> MATLAFILYKYFPFGGLQRDFMRIALECQR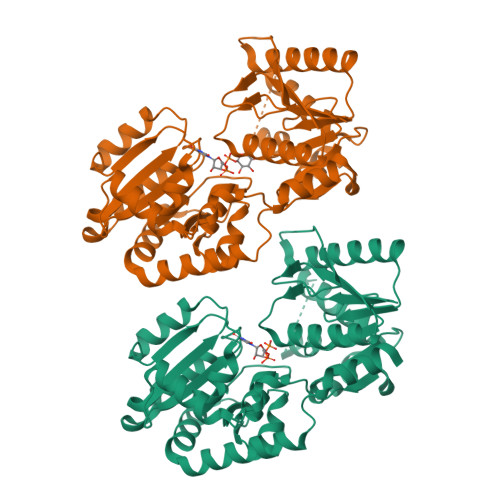RGHDIRVYTLIWEGDVPDGFEVLVAPVRSIFNHRRNEKFTAWVRADLDRRPVQRVIGFNKMPGLDVYYAADACFEEKAQTLRNPLYRQWGRYRHFAGYERAVFDPASKTEILMISEVQQPLFVKHYGTQAERFHLLPPGISQDRRAPANAADVRAEFRREFGLEEDDLLLVQIGSGFKTKGLDRSLKALSALPKALRRRTRLIAIGQDDPKPFLLQIAALGLNDQVQILKGRSDIPRFLLGADLLIHPAYNENTGTVLLEALVSGLPVLVTDVCGYAHYIAEADAGRVLPSPFEQDSLNRLLAEMLEDAPARAAWSRNGLAYADHADLYSMPQRAADLILGEAS;> ATLAFILYKYFPFGGLQRDFMRIALECQRRGHDIRVYTLIWEGDVPDGFEVLVAPVRSIFNHRRNEKFTAWVRADLDRRPVQRVIGFNKMPGLDVYYAADACFEEKAQTLRNPLYRQWGRYRHFAGYERAVFDPASKTEILMISEVQQPLFVKHYGTQAERFHLLPPGISQDRRAPANAADVRAEFRREFGLEEDDLLLVQIGSGFKTKGLDRSLKALSALPKALRRRTRLIAIGQDDPKPFLLQIAALGLNDQVQILKGRSDIPRFLLGADLLIHPAYNENTGTVLLEALVSGLPVLVTDVCGYAHYIAEADAGRVLPSPFEQDSLNRLLAEMLEDAPARAAWSRNGLAYADHADLYSMPQRAADLILG> GPSAGEGGSAAAAPPEVLPTLREWQGGQGEFTLTDRAGIVLDGVRDSRTAADARRFAGELNGKASVSQGRAARPGDIVLRQDPAQKGLLGAEGYRLTVGTRITVTAATSTGVFYGTRTVLQLLNDDGRAARGSATDVPAYRERGVGVCACYINISTQWFERLMKDMASQKLNQLWIEAKVKSDTDPASAFWGYYTKPQVRTLVAMARKYHIELVPEINSPGHMDTYLENHPELQLKDRDGVASPPRLDISRPEALAYYTSMVDEALKVWDSRYWHMGADEYMIGSSYPDYPQLQAAARAKFGASATPDDLFTDFINQVNAHVKADGRSLRIWNDGLAGKNAVVPLDRDITVEHWLSGGSIQQ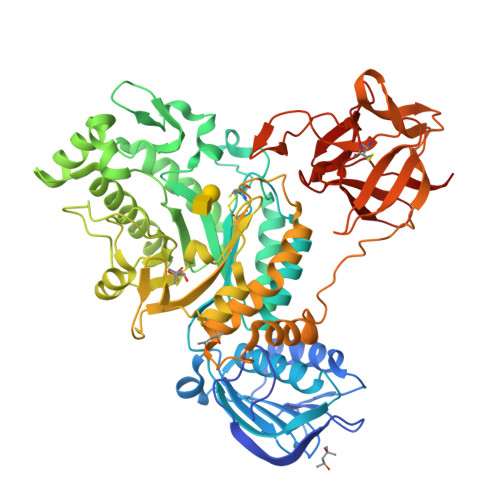PSSLLAEGRPVMNSAYSLYLVRGGFTMQTQKLYESDWTPLRFEGQTLTQGAANLTGAKISLWPDSAAAETENEVETKVFMPLRFVAQATWGGPKPSPTYAGFEALARKIGHAPGWENTDRTPLADGTYRLTTGAKALAPTADAGVSLVKNSAASWALTATADGYYTVRSTESGQCLDAVRGKKYLGAPLEVGAELSLANCSTTARTQRWQLDTGAGALTLRNAISQLHLTERASDGAAVQTTGATRLTARAA> MASTGETTYKKTTSSALKGAIQLGITHSVGSLSQKPERDVLMQDFEVVESIFFPSQGSSSTPGHHHGDFKFKTYAPIAFRYFREMFGIRPDDYLYSLCNEPLIELSNPGASGSLFYVSSDDEFIIKTVQHKEAEFLQTLLPGYFMNLNQNMRTLLPKFYGLYCVQADGKNIRIVVMNNLLPRAVPMHLKFDLKGSTYKRRASPKERSKGVPTYKDLDFMQDMPEGILLENDHYTALSRTMQRDCRVLQSFKIMDYSLLVGIHILHRAGEEASTAVPDTQKKGQGQKPLYCTAIESIQGESKSKTSPQPYESMGGIPAFNSKGERLLVFIGIIDILQSYRLVKKLEHSWKALLHDGDTVSVHRPSFYADRFQKFMCSTVFRKSQLKTLEHHHHHH

The reaction catalysed by the type I PIPK, or phosphatidylinositol 4-phosphate 5-kinase (PIP5K1), is the major synthetic route for PtdIns4,5P2 in most cells. To help elucidating the mechanism for PIP5K1 regulation by DVL, we determine the X-ray structure of the kinase domain of zebrafish PIP5K1A. In this work, we present the first crystal structure of a PIP5K1 molecule. More importantly, the new crystal structure enables us to delineate two adjacent interfaces for dimerization and interaction with DVL that are unique to the PIP5K1 kinases and unravel the importance of these interfaces in regulation of the kinase enzymatic activity by dimerization and interaction with DVL.

The locations of Lys-171 (from the conserved ‘IIK' motif), Asp-299 (MDYSL) and Asp-378 (IID) in the three-dimensional structure of PIP5K1A suggest that they are functionally equivalent to Lys-72, Asp-166 and Asp-184 of PKA, which participate in ATP binding and catalysis. In PIP5K1A, the turn between β8 and α4c is compact. The side chain of Arg-244 is potentially hydrogen bonded to the main chain carbonyl oxygen and side chain carboxylate group of Asp-236, and pushes the side chain of Lys-238 into the active site. Size-exclusion chromatography/multi-angle laser light scattering (SEC/MALLS) indicates that the kinase has a molecular weight of 90 kDa, suggesting that the protein is dimeric in the solution. The crystal structure reveals that the dimer has a side-to-side arrangement, involving both N- and C-lobes of the kinase. Most residues constituting the dimeric interface are found within three structural elements: the loop between α1 and α1a, α4b, and α6. α4b is near the centre of the dimer, and interacts with its symmetric mate (α4b*) through hydrophobic contacts mediated by Pro-186, Phe-189 and Met-190. The negatively charged Asp-84* from the α1*–α1a* loop is matched against a positively charged patch (Arg-287) on α6, while Leu-86* forms hydrophobic contact with Val-291. Unfortunately, the specificity loop (zPIP5K1A residues 386–401), in which the primary determinant of substrate specificity lies28, is disordered in the PIP5K1A structure as in the PIP4K2B structure (Rao et al.), and therefore it remains difficult to rationalize the preferences of PIPKs towards different lipid substrates.> AVNRLQHHHHHHHLEGTVTTDGADIVIKTKGGLEVATTDKEFSFKLGGRLQADYSRFDGFYTKNGNTADAAYFRRAYIELGGTAYKDWKYQINFDLSHNTGSSDNGYFDEASVTYTGFNPVNLKFGRFYPDFGLEKATSSKWVTAPERNAAYELADWINTHQDGMGAQVNSTLADMAYLSAGVSAKDADDSDGDSVKQFNFRGVFAPMHEAGNVLHVGVNYAYRD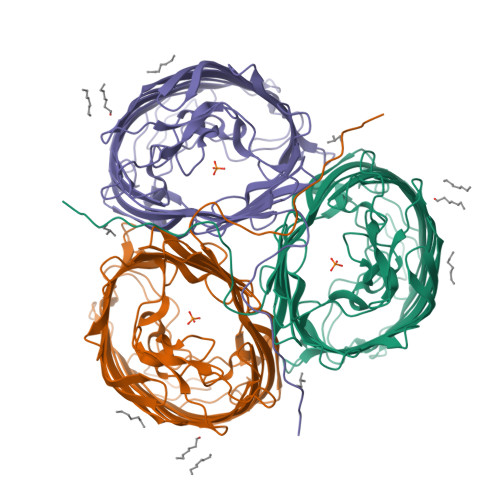LDDTAFDSRIRPRLGMRGIATSGGNDAGDNGNRATFGGVSNSPAGSYKDDSVWGLEGAWAMGPFSAQAEYLARKLKADDNAYKDIKAKGYYAQLAYTLTGESRQYKLEGAKFDSVKPENKEIGAWEVFYRYDNIKVEDDNVVADTATREVGDTKAKAHNLGVNWYVNDAVKISAAYVKAKTDKITNNNGDDDGDGFVTRLQYVF> MSLRPCFVSLIDESDKPILIYVPNEAENEMNDVLKYNVLSNISLDYFESALVEWHSLDSKPLLKSIFQLEGVSVFAMLIKQTGLKIVIGFEQKSLSGADDEFEAINQIFETVRKIYI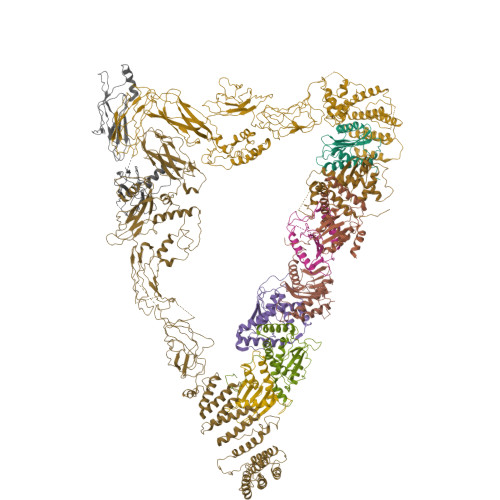RVKCNPLLVSGDEKSIIKSLERKFDELFISTEVEL;> MSSTHSNNVGHPQSSPQGPLTEQQRAQQQYQIFENSLPKVSQSVYQMLLNEMVPLAMGIERQISGDVISSDSNVTSENGNINNMIKRLKIEEHHTVDIIRSHNLIHELYKADEEEKEKVLARLRNIGFQIGLKLSELLIFSNNPNLKFKEMDLLLIMKFICRDVWKQIFGKQIDNLKTNHRGTFYLLDYDYRPIQSFSLEEDAKNEELKMIEPFLEIPVGIIRGVLSSLGYSSEEVICLASFIDRPTDRPKTAFPKGVSFHVQVTMPQ;>[2x]MVSTTQSRSLKAMGEEIWKNKTEKINTELFTLTYGSIVAQLCQDYERDFNKVNDHLYSMGYNIGCRLIEDFLARTALPRCENLVKTSEVLSKCAFKIFLNITPNITNWSHNKDTFSLILDENPLADFVELPMDAMKSLWYSNILCGVLKGSLEMVQLDCDVWFVSDILRGDSQTEIKVKLNRILKDEIPIGED;> MGIYSFWIFDRHCNCIFDREWTLASNSASGTINSKQNEEDAKLLYGMIFSLRSITQKLSKGSVKNDIRSISTGKYRVHTYCTASGLWFVLLSDFKQQSYTQVLQYIYSHIYVKYVSNNLLSPYDFAENENEMRGQGTRKITNRNFISVLESFLAPMVNQ;> MAIETILVINKSGGLIYQRNFTNDEQKLNSNEYLILASTLHGVFAIASQLTPKALQLTQQTNIENTIPYIPYVGMSSNRSDTRNGGGNNNKHTNNEKLGSFKGDDFFKEPFTNWNKSGLRQLCTDQFTMFIYQTLTGLKFVAISSSVMPQRQPTIATTDKPDRPKSTSNLAIQIADNFLRKVYCLYSDYVMKDPSYSMEMPIRSNLFDEKVKKMVENLQ;> MSQRIIQPSASDQQFPGKSDGYEYTVGPKQAITSEASTTYYISRIYSESLLFKRQEASLSAMAFLFQEMISQLHRTCKTAGDFETKLSDYGHNIGIRLLELLNFRASVSPSSLPRASAFLSQNESSSKLSNASNSPGMLANSSTATSASANERLQEKQTESLSNYITKMRRRDLKILDILQFIHGTLWSYLFNHVSDDLVKSSERDNEYMIVDNFPTLTQFIPGENVSCEYFVCGIIKGFLFNAGFPCGVTAHRMPQGGHSQRTVYLIQFDRQVLDREGLRFG;> MPQYFAIIGKKDNPVYEIEFTNAENPQGFPQDLKELNPFILHASLDIVEDLQWQINPTSQLNGNGGNGSNGGGGFLRSRAVNNTDNCYLGKVDHFYGLAITAYISYSGMKFVMIHGNSANSSVVIDDNNMRSFYQEVHELYVKTLMNPFYKITDPIRSPAFDSRVRTLARKHLSK;> MDKEIYCGSVPVSYFDPFDLFESLRPEFQQILPLDNIHWKAFDGTVRTVNRLPIELIPEGRGEADKSNDEQPFIRFLIVNCISIDQYRAKVRPLVRQWLPNLESVSSSTGEKMIYKPIILLYANSEVVDSNLFKSVSLMEKFGKDFPHVQTLEVRSVYRSPKERQEFWNQFSQKIKASVLSIFQKRLTHLQHSLANLQKGNNFEEQLLTREKLYELYVVFNILEDASLELQKIKKEILRRNMNMPDGKLQVPFESSSKSDESLGSIIIEGTLDKFQLHKYFFIRRLRLLKLEDQTLTAFVGAFQLIKNFIESISIEYRKSVRLLEFKHYFITSMLSYFEFENVSNPLLCEIKAELLMLKRDNWVQGVMATSGYRLMDKNYPNSDVKYKFDLLKETFVDETVFQENFLTLTKEILSLFNKCEGKRQRIVDILSIEIGLLYYQGKKYEEAVSLFLSCYEYYTQTNWNSIGLKILQVFIDSLSHCPKLDVLQIDGESVSASAVLTNAFLNILKLCKDNDSKEIWWKKFMDLQMKNNIHLMYPLDGLFEVTLNSKVHLARANVSAIEVNLKSYGFPEDISTKTMRLSLKNMGGDVIVFGASDFLLKKGENKLILECRDIMYGEFSLLSFEIIVEGITFVKEFPENQDEFIVVPEIYCKESTKVLVKQAHNLNLGEYALELKSVQSDALESLQVEVEVQKNIGNMKNLPVSFSMDEIQARKRYNTPFENVRLEYYLLDQITAFDLIIKTSFTKKNDQGTFGETKKVRIQCYLQLSVSVEDIFKKDIFFFKFLLNSSVREEPVILYSSELSAPDTRNDYNIRGDYIATTPALITFDGNESFINCYEITANNNFDSKDIFNLKVRYNTLKEQLDCFITDAVLIEGDVEWFILFEKWKTFWELEILKKLKYDYDAFKENRIIRLLKTSIDLNKTKSKIRNLCIEKAVLDKILICLNKVSRGIAVCNTDMDEYVRNLVPKQLTVPVQLPGFEQFFHVQFEQMETSHDALHDTIATIGNSLSYTVIVENLSGQWGQDVIDDGGYIFEILSSNEWLIHGQKRCAIKEKRKEFEVHLIPLKKGYLNFPRVEITNINGKSCRVDHSNAFESILIF;> MNILKHFPSYVGPSKIRTLVIPIGHWTRKEFNNAVQKLSEFNEIHLSDVTPIDSPIFTPQGFPHGKLFFDFLTIDHDDALELFLYDFEPFRKTFVIIGLVNDYSDPLTNLNFMKEKYPTLISPNLVYASSTPTKELEQTIDTMENVFASSPDMQKNIETIMCDIARNFLTALNSYYSSYKHVTLRSPGAIGGNAVLKTTLIRQNSYTSSSSSTPMSAVQSSVSSSSKAGSVTTASKRLSSFEMTTNSLKRSASLKLATTLSTSENRSQQKSLGRQMKILGNFQLLAGRYVDALNSFVDAITTLYKVRDYLWLGSALDGISICFLLLSYLGLSYQIPQIVSLICPVEKLNFESSSTGISPVDSNSKATASTTASSTPRNSISIAAMQSPRNSIMSLSAPALNIDVENINLPLLIKCISDKVLYYYDLSLMHNSEYAPQVVYCEFLLKTLTFMTSCYKSSEFSKDVLDNIVKNQHRALSDIPNSPMFPRFEVYFYSNKLFELQLKEMQVEAQIKIYSTMAEVYRLLGYKRKQLFVLRLLMVALLATPNKIAWHPDYRTLIDTIIELLNINESEAKINVDDPSQSTWLILQKKILQLCIKVSRKINDFEYVAKFSSILITKYTHLLNQSEQDALFKEYIQPSITNESITSYWDPFILREVVINRILDSDPTSNEIPLESDVSSLESLENRQKTQDINPQEVFNPFKRVQPTSFVSNNSTKVPILVFLVGDKAEFTCRVQNPFKFDFTINDIQLDEEISEFCEIDRKAVSYSGPYNVKAESIRSITLPLIIKKPTYKKIYEISCLKISILKLPLQKFDIINDSRRSNPVEEEAEYSKCIYGKLKIKILPEQPQLELLSTSKMTRNSWMMLDGTKTDFHITVRNKSLSCAINHIKIIPMNNIEQMLKPDYWKKMPPDDLYIMEKQLDWLSKSCVRIIKLPTVIKPNETITFDLELDNTAVPFNFTGFDLLIEYGMSATDESCIYLKKLSIPYEVTLRRTIEVPSMDIIPLNELFSSQVENVDWIEYVMSKIRAESNLHSRDFILLLLDFRNSWIDGIKLNVQFEDFTSNEYHVEASHTSRIIVPIKKIDYKKYNFENTPIPRIYPGRQFIQSGLNEEQTIEMRQKFWCREHIISKLKCNWKLTTDQSVTGSVDFNKFIEKFDHKMVYTIYPGRLFYGVQLLLDEPKVKVGEIINLKIITEPTSTCRRKQNSTVNFLDIVIFDSKTSKILPRSNRRILYNGSLTKPISTTKVSEINLEIIPIEKGRYEFSVCISKSNNQDGIIQFDSENVILSVI;> MECFVPLRCDLDGSNIEQLRQSHLSRKFIIFDEQLNLWLWFQGNSQENKRFVLQNMIILINEAQVTRTSTIDDYFTQVENNENLWRLKNDCCSKILFKSNVVMNNGYNNQIKFVFEYKSVDANFNNQDSLQDPQAKYTLDKYSSEEILPSFEPVYSWSSAATKSSKNTNNHLEKNNRATHRVSSKNSEVHEADVSRNPNTFTLKLQYPIFSLLNMRLRNISLKSEHCILSSLDFQTSKASEQLTKKFIYPQEHNSFLKLNFQEISYKLIDGTSQIELDPICPLKVPLTAFSYDSISATFKLVLLPKSTQPHRVKITLAYELELHPNLKLPVRTSWETEVTLKRSMPISSTSSQYSSNNNNTNHSASFNGAANNVNSGGLANLRLGGVSSSRFSLGAASTTSLVNSKLSNVKFKFINSNIKVIKGEKFTMRLQIINSSSSPLDLVVYYNNTINPIPSANNVRNSNGINNCGMNNGTIPNSPLTLENQYQLHNKYRKIAEGIILLSNDYKIPVVPPRETYFADLRFIGIMSGYYGTLSGLKVLDLNTNELIEVGNGASVLI Crystal structures are presented for a putative uncharacterized protein that shares sequence similarity with ζ-class glutathione S-transferases (GSTs) in both apo and glutathione-bound forms. Each protomer consists of an N-­terminal βαβαββα thioredoxin-like fold common to all GSTs as well as a C-­terminal α-helical domain. Based on sequence homology, structural similarity, half-site glutathione binding and sulfate ion H-site binding, the protein investigated here is likely to be a ζ-class GST/MAAI. Glutathione S-transferases (GSTs) are detoxifying enzymes that appear across a wide range of aerobic organisms, including bacteria, fungi, plants and mammals.

A 1.85 Å resolution crystal structure was determined from a crystal grown in the presence of 10 mM glutathione (∼10.7 equivalents relative to protein at 0.93 mM). The structure was of a different crystal form to the apo structure and contained one dimer in the asymmetric unit. This structure revealed the presence of glutathione in one protomer, again revealing a nonsymmetrical dimer. The glutathione-bound protomer was ordered from residues 3 to 230, whereas the other unliganded protomer was ordered from residues 3 to 39 and residues 55 to 231. The distance between the Cys16 S atom and the glutathione S atom was 3.7 Å. A sulfate ion was observed in the same position off Ser14 as in the apo crystal structure, again with Arg190 positioned away from the sulfate ion (4.6 Å). Considerable movement of some components of the active site relative to the glutathione-free form was observed, indicating an induced-fit mechanism for cofactor binding. In the C. immitis structure glutathione is bound in only one half-site. This is consistent with binding studies on human GSTZ1-1, which showed half-site glutathione binding even at saturating glutathione concentrations and are suggestive of a cooperative mechanism.

>[2x]GPGSMTTPNFELYGYFRSSCSGRLRIAFHLKSIPYTRHPVNLLKGEQHSDTYKSLNPTNTVPLLVVSNINNTVSPSSASFSIGQSLAALEYLEEALPTNARPLLPPISNPVARAHVRTICNIIACDVQPVTNLKIQKKVKALDGDPTVWSRDLATQGFGAVEKLLELSAGRFCVGDEITLADVCLVPAVWAAERVGMDLARFPITKRVFEEMLKEEAVQKAHWQKQEDTPEDLRA>[4x]MKILKTLTLRGPNYWSIRRKKLIVMRLDLEDLAERPSNSIPGFYEGLIKVLPSLVEHFCSPGYQGGFLERVKEGTYMGHIVEHVALELQELVGMTAGFGRTRETSTPGVYNVVYEYVDEQAGRYAGRAAVRLCRSLVDTGDYPRLELEKDLEDLRDLGANSALGPSTETIVTEAEARKIPWMLLSARAMVQLGYGVYQQRIQATLSSHSGILGVELACDKEGTKTILQDAG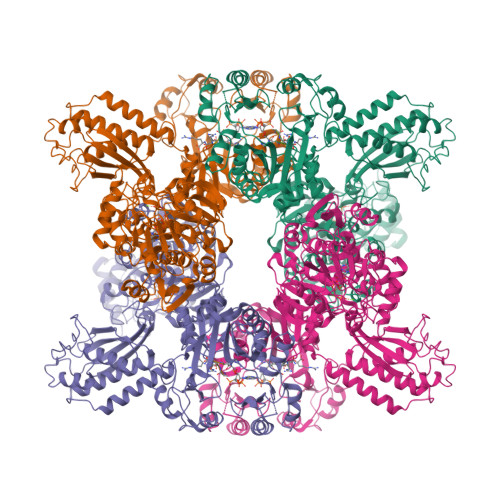IPVPRGTTIQYFDDLEEAINDVGGYPVVIKPLDGNHGRGITINVRHWQEAIAAYDLAAEESKSRAIIVERYYEGSDHRVLVVNGKLVAVAERIPAHVTGDGSSTISELIEKTNQDPNRGDGHDNILTKIVVNKTAIDVMERQGYNLDSVLPKDEVVYLRATANLSTGGIAIDRTDDIHPENIWLMERVAKVIGLDIAGIDVVTSDISKPLRETNGVIVEVNAAPGFRMHVAPSQGLPRNVAAPVLDMLFPPGTPSRIPILAVTGTNGKTTTTRLLAHIYRQTGKTVGYTSTDAIYINEYCVEKGDNTGPQSAGVILRDPTVEVAVLETARGGILRAGLAFDSCDVGVVLNVAADHLGLGDIDTIEQMAKVKSVIAEVVDPSGYAVLNADDPLVAAMADKVKAKVAYFSMNPDNPIIQAHVRRNGIAAVYESGYLSILEGSWTLRVEQAKLIPMTMGGMAPFMIANALAACLAAFVNGLDVEVIRQGVRTFTTSAEQTPGRMNLFNLGQHHALVDYAHNPAGYRAVGDFVKNWQGQRFGVVGGPGDRRDSDLIELGQIAAQVFDRIIVKEDDDKRGRSEGETADLIVKGILQENPGASYEVILDETIALNKALDQVEEKGLVVVFPESVTRAIDLIKVRNPIGENLYFQ;>[4x]DDDDDDDDX> DSIVVAYYFCGEPIPDRTLVRGRAVTLGQFKEL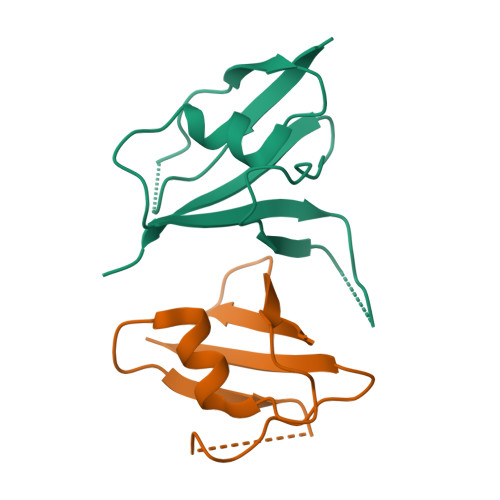LTKKGSYRYYFKKVSDEFDCGVVFEEVREDEAVLPVFEEKIIGKVEKVD;> GETKVIYHLDEEETPYLVKIPVPAERITLGDFKSVLQRPAGAKYFFKSMDQDFGVAAEEISDDNARLPCFNGRVVSWLVSSD>SSEQLKHCNGILKELLSKKHAAYAWPFYKPVDASALGLHDYHDIIKHPMDLSTVKRKMENRDYRDAQEFAADVRLMFSNCYKYNPPDHDVVAMARKLQDVFEFRYAK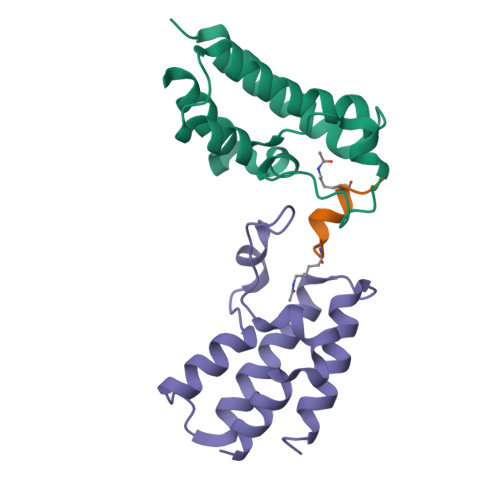MP[8x];>[4x]XWKGYLCLRKRIQ> ALAPRQVLDLEDLVFTQGSHFMANKRCQLPDGSFRRQRKGYEEVHVPALKPKPFGSEEQLLPVEKLPKYAQAGFEGFKTLNRIQSKLYRAALETDENLLLCAPTGAGKTNVALMCMLREIGKHINMDGTINVDDFKIIYIAPMRSLVQEMVGSFGKRLATYGITVAELTGDHQLCKEEISATQIIVCTPEKWDIITRKGGERTYTQLVRLIILDEIHLLHDDRGPVLEALVARAIRNIEMTQEDVRLIGLSATLPNYEDVATFLRVDPAKGLFYFDNSFRPVPLEQTYVGITEKKAIKRFQIMNEIVYEKIMEHAGKNQVLVFVHSRKETGKTARAIRDMCLEKDTLGLFLREGSASTEVLRTEAEQCKNLELKDLLPYGFAIHHAGMTRVDRTLVEDLFADKHIQVLVSTATLAWGVNLPAHTVIIKGTQVYSPEKGRWTELGALDILQMLGRAGRPQYDTKGEGILITSHGELQYYLSLLNQQLPIESQMVSKLPDMLNAEIVLGNVQNAKDAVNWLGYAYLYIRMLRSPTLYGISHDDLKGDPLLDQRRLDLVHTAALMLDKNNLVKYDKKTGNFQVTELGRIASHYYITNDTVQTYNQLLKPTLSEIELFRVFSLSSEFKNITVREEEKLELQKLLERVPIPVKESIEEPSAKINVLLQAFISQLKLEGFALMADMVYVTQLAGRLMRAIFEIVLNRGWAQLTDKTLNLCKMIDKRMWQSMCPLRQFRKLPEEVVKKIEKKNFPFERLYDLNHNEIGELIRMPKMGKTIHKYVHLFPKLELSVHLQPITRSTLKVELTITPDFQWDEKVHGSSEAFWILVEDVDSEVILHHEYFLLKAKYAQDEHLITFFVPVFEPLPPQYFIRVVSDRWLSCETQLPVSFRHLILPEKYPPPTELLDLQPLPVSALRNSAFESLYQDKFPFFNPIQTQVFNTVYNSDDNVFVGAPTGSGKTICAEFAILRMLLQSSEGRCVYITPMEALAEQVYMDWYEKFQDRLNKKVVLLTGETSTDLKLLGKGNIIISTPEKWDILSRRWKQRKNVQNINLFVVDEVHLIGGENGPVLEVICSRMRYISSQIERPIRIVALSSSLSNAKDVAHWLGCSATSTFNFHPNVRPVPLELHIQGFNISHTQTRLLSMAKPVYHAITKHSPKKPVIVFVPSRKQTRLTAIDILTTCAADIQRQRFLHCTEKDLIPYLEKLSDSTLKETLLNGVGYLHEGLSPMERRLVEQLFSSGAIQVVVASRSLCWGMNVAAHLVIIMDTQYYNGKIHAYVDYPIYDVLQMVGHANRPLQDDEGRCVIMCQGSKKDFFKKFLYEPLPVESHLDHCMHDHFNAEIVTKTIENKQDAVDYLTWTFLYRRMTQNPNYYNLQGISHRHLSDHLSELVEQTLSDLEQSKCISIEDEMDVAPLNLGM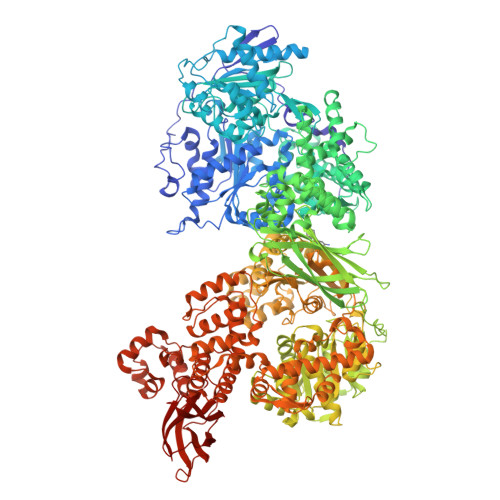IAAYYYINYTTIELFSMSLNAKTKVRGLIEIISNAAEYENIPIRHHEDNLLRQLAQKVPHKLNNPKFNDPHVKTNLLLQAHLSRMQLSAELQSDTEEILSKAIRLIQACVDVLSSNGWLSPALAAMELAQMVTQAMWSKDSYLKQLPHFTSEHIKRCTDKGVESVFDIMEMEDEERNALLQLTDSQIADVARFCNRYPNIELSYEVVDKDSIRSGGPVVVLVQLEREEEVTGPVIAPLFPQKREEGWWVVIGDAKSNSLISIKRLTLQQKAKVKLDFVAPATGAHNYTLYFMSDAYMGCDQEYKFSVD>[3x]GSTPADVKEHPNSYVFMVDMPGVKSGDIKVQV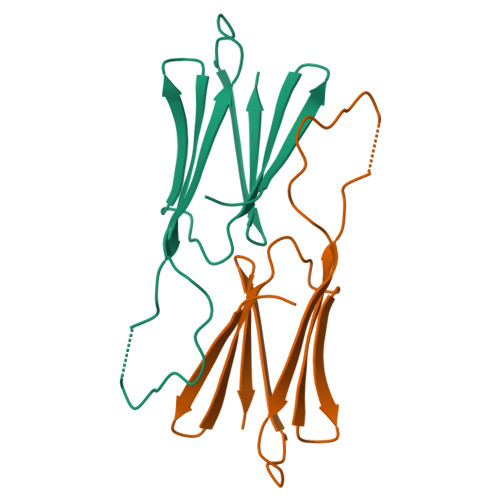EDENVLLISGERKREEEKEGVKYLKMERRIGKLMRKFVLPENANIEAISAISQDGVLTVTVNK>[2x]MSETSRTAFGGRRAVPPNNSNAAEDDLPTVELQGVVPRGVNLQEFLNVTSVHLFKERWDTNKVDHHTDKYENNKLIVRRGQSFYVQIDFSRPYDPRRDLFRVEYVIGRYPQENKGTYIPVPIVSELQSGKWGAKIVMREDRSVRLSIQSSPKCIVGKFRMYVAVWTPYGVLRTSRNPETDTYILFNPWCEDDAVYLDNEKEREEYVLNDIGVIFYGEVNDIKTRSWSYGQFEDGILDTCLYVMDRAQMDLSGRGNPIKVSRVGSAMVNAKDDEGVLVGSWDNIYAYGVPPSAWTGSVDILLEYRSSENPVRYGQCWVFAGVFNTFLRCLGIPARIVTNYFSAHDNDANLQMDIFLEEDGNVNSKLTKDSVWNYHCWNEAWMTRPDLPVGFGGWQAVDSTPQENSDGMYRCGPASVQAIKHGHVCFQFDAPFVFAEVNSDLIYITAKKDGTHVVENVDATHIGKLIVTKQIGGDGMMDITDTYKFQEGQEEERLALETALMYGAKKPLNTEGVMKSRSNVDMDFEVENAVLGKDFKLSITFRNNSHNRYTITAYLSANITFYTGVPKAEFKKETFDVTLEPLSFKKEAVLIQAGEYMGQLLEQASLHFFVTARINETRDVLAKQKSTVLTIPEIIIKVRGTQVVGSDMTVTVEFTNPLKETLRNVWVHLDGPGVTRPMKKMFREIRPNSTVQWEEVCRPWVSGHRKLIASMSSDSLRHVYGELD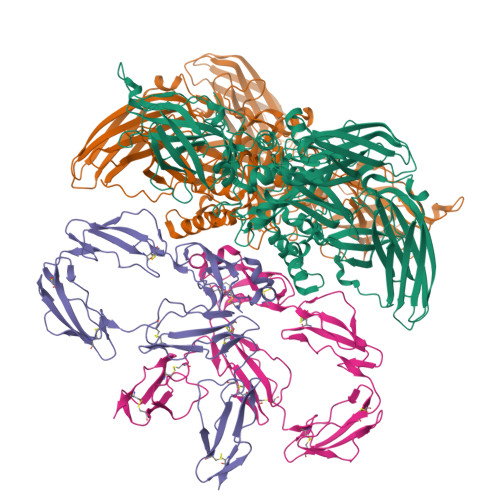VQIQRRPSM;>[2x]MRLKNLTFIIILIISGELYAEEKPCGFPHVENGRIAQYYYTFKSFYFPMSIDKKLSFFCLAGYTTESGRQEEQTTCTTEGWSPEPRCFKKCTKPDLSNGYISDVKLLYKIQENMRYGCASGYKTTGGKDEEVVQCLSDGWSSQPTCRKEHETCLAPELYNGNYSTTQKTFKVKDKVQYECATGYYTAGGKKTEEVECLTYGWSLTPKCTKLKCSSLRLIENGYFHPVKQTYEEGDVVQFFCHENYYLSGSDLIQCYNFGWYPESPVCEGRRNRCPPPPLPINSKIQTHSTTYRHGEIVHIECELNFEIHGSAEIRCEDGKWTEPPKCIEGQEKVACEEPPFIENGAANLHSKIYYNGDKVTYACKSGYLLHGSNEITCNRGKWTLPPECVENNENCKHPPVVMNGAVADGILASYATGSSVEYRCNEYYLLRGSKISRCEQGKWSSPPVCLEPCTVNVDYMNRNNIEMKWKYEGKVLHGDLIDFVCKQGYDLSPLTPLSELSVQCNRGEVKYPLCTRKESKGMCTSPPLIKHGVIISSTVDTYENGSSVEYRCFDHHFLEGSREAYCLDGMWTTPPLCLEPCTLSFTEMEKNNLLLKWDFDNRPHILHGEYIEFICRGDTYPAELYITGSILRMQCDRGQLKYPRCIPRQSTLSYQEPLRT> TVVEEPVDITPYLDQLDESLRDKVLQLQKGSDTEAQCEVMQEIVDQVLEEDFDSEQLSVLASCLQELFKAHFRGEVLPEEITEESLEESVGKPLYLIFRNLCQMQEDNSSFSLLLDLLSELYQKQPKIGYHLLYYLRASKAAAGKMNLYESFAQATQLGDLHTCLMMDMKACQEDDVRLLCHLTPSIYTEFPDETLRSGELLNMIVAVIDSAQLQELVCHVMMGNLVMFRKDSVLNILIQSLDWETFEQYCAWQLFLAHNIPLETIIPILQHLKYKEHPEALSC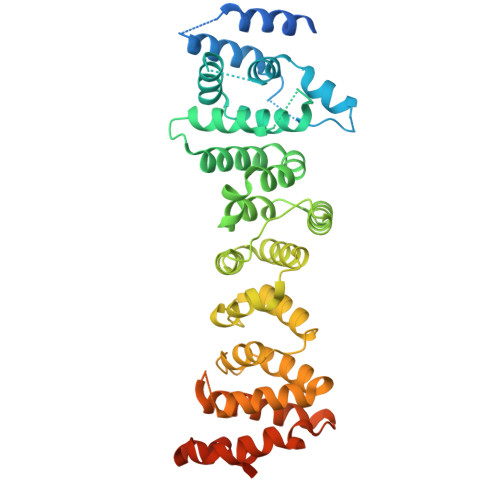LLLQLRREKPSEEMVKMVLSRPCHPDDQFTTSILRHWCMKHDELLAEHIKSLLIKNNSLPRKRQSLRSSSSKLAQLTLEQILEHLDNLRLNLTNTKQNFFSQTPILQALQHVQASCDEAHKMKFSDLFSLAEEYEDSSTKPPKSRRKAALSS> MSLRRGIYHIENAGVPSAIDLKDGSSSDGTPIVGWQFTPDTINWHQLWLAEPIPNVADTFTLCNLFSGTYMDLYNGSSEAGTAVNGWQGTAFTTNPHQLWTIKKSSDGTSYKIQNY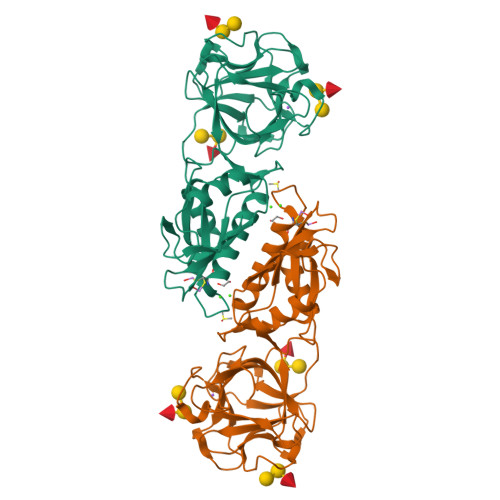GSKTFVDLVNGDSSDGAKIAGWTGTWDEGNPHQKWYFNRMSVSSAEAQAAIARNPHIHGTYRGYILDGEYLVLPNATFTQIWKDSGLPGSKQREQIYDCDDFAIAMKAAVGKWGADSWKANGFAIFCGVMLGVNKAGDAAHAYNFTLTKDHADIVFFEPWNGGYLNDIGYDSYMAFY RNA ligases of the RTCB-type play an essential role in tRNA splicing, the unfolded protein response and RNA repair. RTCB is the catalytic subunit of the pentameric human tRNA ligase complex. RNA ligation by the tRNA ligase complex requires GTP-dependent activation of RTCB. This active site guanylylation reaction relies on the activation factor Archease.

Co-crystallizing with Mn2+ and the non-hydrolyzable GTP analog GMPCPP allowed us to obtain an RTCB-Archease complex with a well-resolved GMPCPP molecule in the active site of RTCB. Strikingly, three Mn2+ ions were bound in the composite active site formed by RTCB and Archease (left). Our complex structures revealed an additional metal site, named position C, which solely depends on Archease residues for Mn2+ binding. Mn2+(A) is octahedrally coordinated by RTCB side chains H259 (e; equatorial), H353 (a; axial), C122 (e), a water molecule (e) and two oxygens from the alpha (e) and beta (a) phosphate moieties of GMPCPP. Mn2+(B) is tetrahedrally coordinated by RTCB side chains D119, C122, H227 and an oxygen atom from the γ-phosphate part of GMPCPP. Mn2+(C) is coordinated octahedrally by Archease side chains D51 (a), D178 (e), the terminal carboxyl group of I179 (e), an oxygen (a) of the γ-phosphate moiety of GMPCPP and two water molecules (e). Moreover, H428Nε2, α-phosphorus atom and carbon atom of GMPCPP are nearly in line, i.e., have adopted already the geometry required for the guanylylation reaction. Overall, the structure mimics a pre-activation state in which Archease is already bound but the guanylyl group is not yet transferred to H428 (left). In both complexes the conserved tip of the arrowhead-shaped Archease is reaching directly into the active site of RTCB, thus forming an extensive interface between both proteins with an area of about 2200 Å2. While the Mn2+ ions in positions A and C are present in both, the pre- and post-activation complex, position B is only occupied by Mn2+ in the pre-activation state.

>[4x]GAMSRSYNDELQFLEKINKNCWRIKKGFVPNMQVEGVFYVNDALEKLMFEELRNACRGGGVGGFLPAMKQIGNVAALPGIVHRSIGLPDVHSGYGFAIGNMAAFDMNDPEAVVSPGGVGFDINCGVRLLRTNLDESDVQPVKEQLAQAMFDHIPVGVGSKGVIPMNAKDLEEALEMGVDWSLREGYAWAEDKEHCEEYGRMLQADPNKVSARAKKRGLPQLGTLGAGNHYAEIQVVDEIFNEYAAKKMGIDHKGQVCVMIHSGSRGLGHQVATDALVAMEKAMKRDKIIVNDRQLACARIASPEGQDYLKGMAAAGNYAWVNRSSMTFLTRQAFAKVFNTTPDDLDLHVIYDVSHNIAKVEQHVVDGKERTLLVHRKGSTRAFPPHHPLIAVDYQLTGQPVLIGGTMGTCSYVLTGTEQGMTETFGTTCHGAGRALSRAKSRRNLDFQDVLDKLADMGIAIRVASPKLVMEEAPESYKNVTDVVNTCHDAGISKKAIKLRPIAVIKG;>GSHMMKGGSRVSNPAVMAQEEEDVRDYNLTEEQKAIKAKYPPVNRKYEYLDHTADVQLHAWGDTLEEAFEQCAMAMFGYMTDTGTVEPLQTVEVETQGDDLQSLLFHFLDEWLYKFSADEFFIPREVKVLSIDQRNFKLRSIGWGEEFSLSKHPQGTEVKAITYSAMQVYNEENPEVFVIIDI[4x]> TAPTLTVTPEQ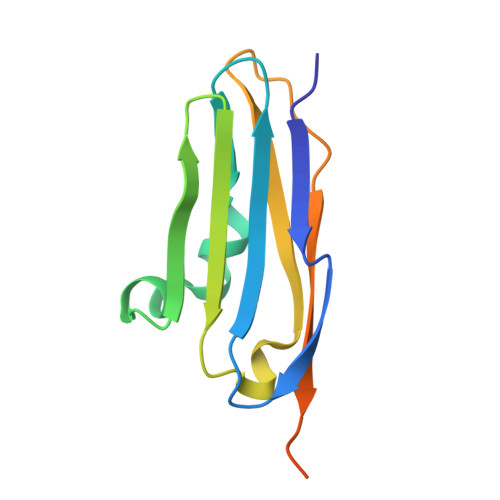QTVKVDEDITFTVTVEDENEVELGLDDLKAKYENDIIGARVKIKYLTKEPNKKVMEVTIMKATLADKGAITFTAKDKAGNQAEPKTVTINVLPLKDSNEPKLPSTGGSHHHHHH>SMRIGANGDETVWADEEFAGRDFRDEDLSRIRTERVVFTECDFSGVDLSESEHHGSAFRNCTFRRSTIWHSTFTNCSLLGSVFTECRIRPVTFVECDFTLAVLGGCDLRAVDLSDCRLREVSLVGADLRKAVLRRADLTGSRVQDARLEEADLRGTRVDPTFWTTAKVRGAKIDIEQAL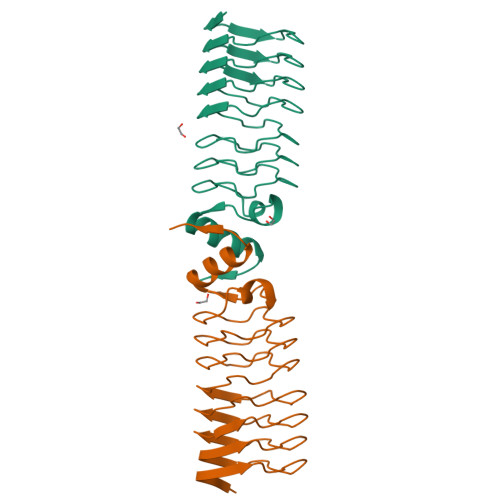AYAAAHGLAVHGG[2x]> MKKKIIIAIVASAITMTHFVGNTYADSKTEVSVTAPYNTNQIAKWLEAHAKPLKTTNPTASLNDLKPLKNMVGSASIVGLGEATHGAHEVFTMKHRIVKYLVSEKGFTNLVLEEGWDRALELDRYVLTGKGNPSQHLTPVFKTKEMLDLLDWIRQYNANPKHKSKVRVIGMDIQSVNENVYNNIIEYIKANNSKLLPRVEEKIKGLIPVTKDMNTFESLTKEEKEKYVLDAKTISALLEENKSYLNGKSKEFAWIKQNARIIEQFTTMLATPPDKPADFYLKH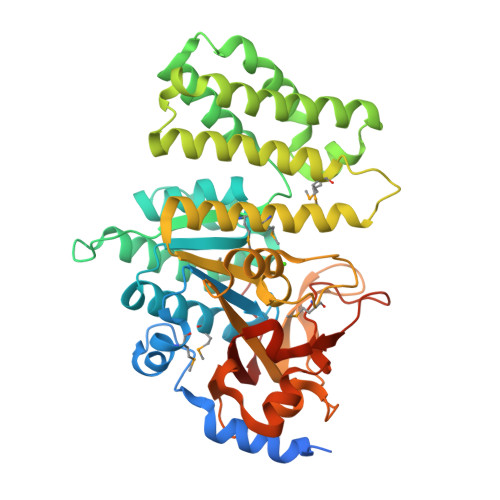DIAMYENAKWTEEHLGKTIVWGHNGHVSKTNMLSFIYPKVAGQHLAEYYGKRYVSIGTSVYEGQYNVKNSDGEFGPYGTLKSDDPNSYNYIFGQVKKDQFFIDLRKANGVTKTWLNEQHPIFAGITTEGPDIPKTVDISLGKAFDILVQIQKVSPSQVHQLEHHHHHH> MGSSHHHHHHSQDPKPRVLVLTGAGISAESGIRTFRAADGLWEEHRVEDVATPEGFDRDPELVQAFYNARRRQLQQPEIQPNAAHL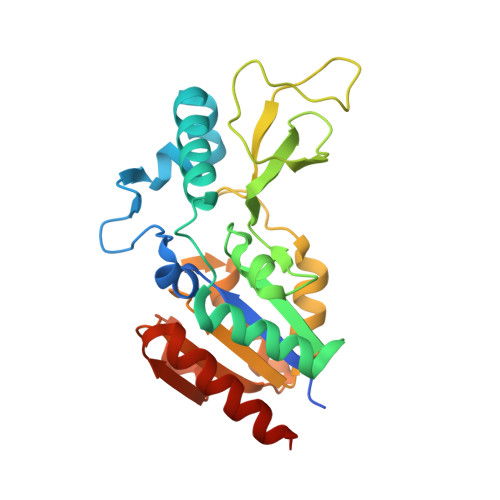ALAKLQDALGDRFLLVTQNIDNLHERAGNTNVIHMHGELLKVRCSQSGQVLDWTGDVTPEDKCHCCQFPAPLRPHVVWFGEMPLGMDEIYMALSMADIFIAIGTSGHVYPAAGFVHEAKLHGAHTVELNLEPSQVGNEFAEKYYGPASQVVPEFVEKLLKGLKAGSIA> MDDLKLPRQRVDLVAPPFVHVHEQATKQGPKIMEFKLVVQEKKMVIDEKGTTFQAMTFNGSMPGPLMVVHEGDYVEVTLVNPATNTMPHNIDFHSATGALGGGALTLINPGEQVVLRWKATRTGVFVYHCAPGGPMIPWHVVSGMNGAVMVLPRDGLNDGHGHSLRYDRIYYIGEQDLYVPRDEKGNFKSYDSPGEAYSDTEEVMRKLTPTHVVFNGKAGALTGKNALNANVGENVLIVHSQANRDSRPHLIGGHGDYVWETGKFSNAPETGLETWFIRGGSAGAALYKFLQPGIYAYVTHNLIEAANLGATAHFKVEGKWNDDLMTQVKAPADIPTGSTNENLYFQGGS

CuNiRs catalyze the conversion of nitrite to gaseous nitric oxide (NO2− + 2H+ + e− → NO + H2O) in the first committed step of the denitrification pathway. The two redox Cu centers are coupled via the neighboring Cys-His residues that form a conserved hard-wired 12.6-Å ET bridge. A two-domain blue CuNiR from a Rhizobia species (Br2DNiR) has recently been structurally characterized showing an unusual oxidized T2CuII-(His)3-(H2O)2 coordination site, requiring the displacement of two water molecules by the substrate instead of a single water molecule in a prototypic CuNiR.

Online optical single crystal spectroscopy has been combined with the MSOX X-ray crystallography approach using a single blue Br2DNiR crystal maintained at 100 K in the as-isolated state (i.e., in absence of nitrite). Optical spectroscopy prior to X-ray irradiation confirmed that the T1Cu site was in its oxidized [CuII] state, as expected from studies with other blue CuNiRs (e.g., AxNiR). A total of 20 crystallographic datasets were obtained from the same spot of the Br2DNiR crystal with a dose of 0.4 MGy per dataset (estimated by RADDOSE-3D(25)). Following exposure to the first dose of X-rays, the optical spectrum showed a clear loss of the optical absorption peak at ∼460 nm and a substantial reduction of the peak at ∼595 nm. A crystallographic MSOX movie of serial structures to a resolution of 1.35 Å while the optical spectra were reporting on the redox status of T1Cu allowed us to define structural changes resulting from the T1Cu radiation-induced chemistry throughout the structure including the catalytic T2Cu site. Data collection and refinement statistics are provided for dataset 1 (DS1), DS5, and DS20 in Table 1 as representatives of the data quality and refinement for the individual structures. The first structure showed two full occupancy water molecules (W1 and W2) coordinated to T2Cu as was previously observed for Br2DNiR, with W1 more closely coordinated. Two conformations of the catalytic Asp residue (Asp92CAT) in its proximal and distorted position are also seen with two conformations of channel water (W4).>MHHHHHHHHHHSETTYTGPRSIVTPETPIGPSSY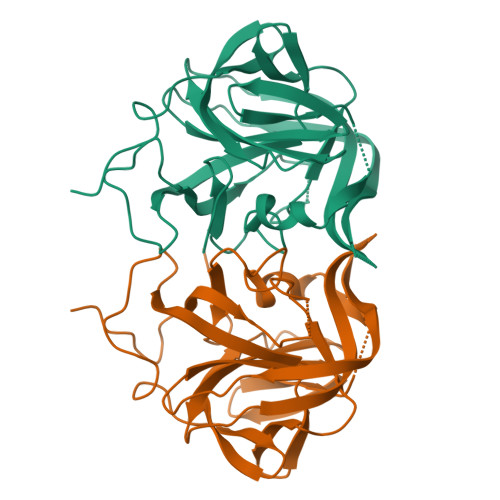PMTPSSLVLMAGYFSGPEISDNFGKYMPLLFQQNTSKVTFRSGSHTIKIVSMVLVDRLMWLDKHFNQYTNEPDGVFGDVGNVFVDNDNVAKVITMSGSSAPANRGATLMLCRATKNIQTFNFAATVYIPAYKVKDGAGGKDVVLNVAQWEANKTLTYPAIPKDTYFMVVTMGGASFTIQRYVVYNEGIGDGLELPAFWGKYLSQLYGFSWSSPTYACVTWEPIYAEEGIPHR[3x]> MSTENRVIDLVVDENVPYGLLMQFMDVDDSVYPSTSKP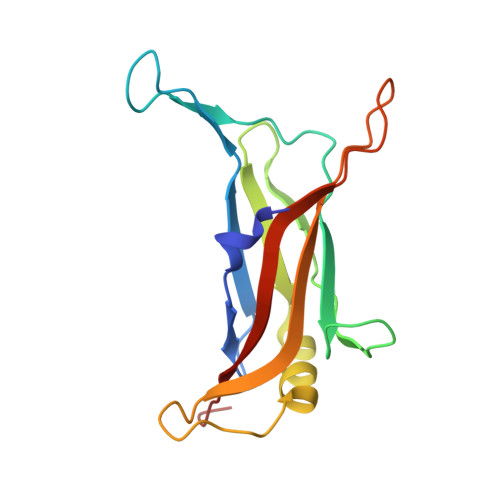VDLTDFSLRGSIKSSLEDGAETVASFTTAIVDAAQGVASISLPVSAVTTIASKASKERDRYNPRQRLAGYYDVIITRTAVGSAASSFRIMEGKVYISDGVTQ> GGSEAVSDIYKPFWEWAAKTIKERLGDDLVSYPIPDGYLRKEAMVGKGKRESLAWTQSYG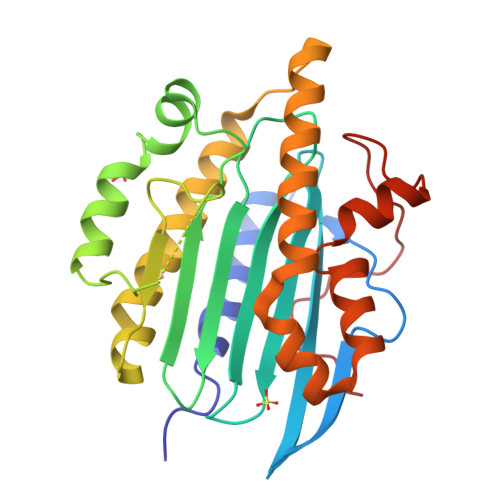YQTKKMRQIRAAHVNGGASLQVLNLVFFPHMNYDLPFLGLDLVTLPGGHLIAIDMQPLFQTEEYKKKYAEPCMDMYQKHVKNLPWGGDFPEEAKQYFSPVFLWTRPQEDKQVETYVFEAFKDYINKYLDFVEAAKPVTDPDHLARIRERQLSYLQYRAEKDPARGMFTRMYGPEWTERYIHGFLFDLEEKMESGEYKTGELLPCSDPLNFQPTPL>EPFWADLQPRVAFVERGGSLWLNCSTNCPRPERGGLETSLRRNGTQRGLRWLARQLVDIREPETQPVCFFRCARRTLQARGLIRTFQRPDRVELMPLPPWQPVGENFTLSCRVPGAGPRASLTLTLLRGAQELIRRSFAGEPPRARGAVLTATVLARREDHGANFSCRAELDLRPHGLGLFENSSAPRELRTFSLSPDAPRLAAPRLLEVGSERPVSCTLDGLFPASEARVYLALGDQNLSPDVTLEGDAFVATATATASAEQEGARQLVCNVTLGGENRETRENVTIY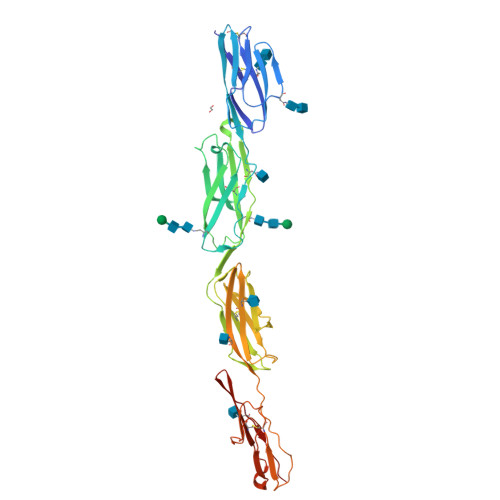SFPAPLLTLSEPSVSEGQMVTVTCAAGAQALVTLEGVPAAVPGQPAQLQLNATENDDRRSFFCDATLDVDGETLIKNRSAELRVLYAPR[2x]> MADSDINIKTGTTDIGSNTTVKTGDLVTYDKENGMHKKVFYSFIDDKNHNKKLLVIRTKGTIAGQYRVYSEEGANKSGLAWPSAFKVQLQLPDNEVAQISDYYPRNSIDTKEYMSTLTYGFNSNVTGDDTGKIGGLIGANVSIGHTLRYVQPDFKTILESPTDKKVGWKVIFNNMVNQNWGPYDRDSWNPVYGNQLFMKTRNGSMKAADNFLDPNKASSLLSSGFSPDFATVITMDRKASKQQ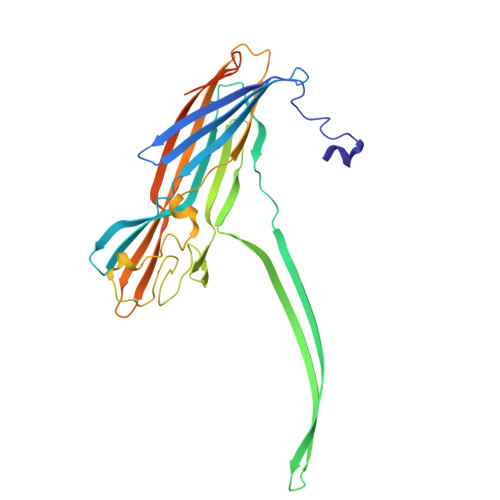TNIDVIYERVRDDYQLHWTSTNWKGTNTKDKWTDRSSERYKIDWEKEEMTNGSSGSRGVPHIVMVDAYKRYKGGSHHHHHH GALK1 is a small molecule kinase of the GHMP kinase family, which catalyzes the MgATP-dependent phosphorylation of the C-1 hydroxyl of α-d-galactose to yield Gal-1-P in the Leloir pathway. In classic galactosemia, GALT enzymatic deficiency causes the accumulation of Gal-1-P, the product of the enzyme galactokinase 1 (GALK1; EC 2.7.1.6) upstream of GALT in the Leloir pathway. Inhibition of human GALK1 (hGALK1) to prevent Gal-1-P production therefore could provide a therapeutic benefit for GALT deficiency. Here, we determined crystal structures of hGALK1 bound with reported ATP-competitive inhibitors of the spiro-benzoxazole series, to reveal their binding mode in the active site.

To this end, we co-crystallized hGALK1 with two spiro-benzoxazole inhibitors (T1 and T2), in the presence of galactose, and determined their crystal structures to 2.44 and 2.10 Å resolution, respectively. T1 and T2 share the chemical scaffold of a benzoxazole ring connected to a tetrahydroquinazolinone ring by an amide linker, and both compounds are found to occupy the ATP binding site in a similar manner. The benzoxazole ring, mimicking the adenine moiety of ATP, sits in a hydrophobic pocket forming a π–π stacking interaction with Trp106 and van der Waals interactions with Val129 and Leu145. Importantly, the quinazolinone cyclohexanone and spiro-ring substituents cause displacement of two key side-chains—Arg105 and Arg228—at the entrance of the ATP site. In our costructures, both Arg105 and Arg228 are sequestered away from the ATP phosphate groups, to accommodate the quinazolinone ring of the compounds. For T2 with the larger spiro ring, the carbonyl moiety is close enough to hydrogen bond with the Arg105 guanidino side chain (dotted line). Therefore, these residues are sequestered away from catalysis in the inhibitor-bound complexes. ATP-titration experiments with T2 showed no significant change in Vmaxapp (P = 0.1801) and a significant increase in Kmapp (P < 0.0001), collectively indicating competitive inhibition with ATP by T2, which is supported by fitting in GraphPad Prism and is in agreement with its binding mode in our hGALK1 crystal costructure. We found that hGALK1 co-crystallized with galactose and T2 produced the required quantity (crystals in the hundreds) and diffraction quality (consistently better than 2.5 Å) for the screening campaign. To bias hits toward allosteric binding, we soaked compounds into hGALK1 co-crystals with galactose and T2 occupying the active site.

>HHAALRQPQVAELLAEARRAFREEFGAEPELAVSAPGRVNLIGEHTDYNQGLVLPMALELMTVLVGSPRKDGLVSLLTTSEGADEPQRLQFPLPTAQRSLEPGTPRWANYVKGVIQYYPAAPLPGFSAVVVSSVPLGGGLSSSASLEVATYTFLQQLCPDSGTIAARAQVCQQAEHSFAGMPCGIMDQFISLMGQKGHALLIDCRSLETSLVPLSDPKLAVLITNSNVRHSLASSEYPVRRRQCEEVARALGAASLREVQLEELEAARDLVSKEGFRRARHVVGEIRRTAQAAAALRRGDYRAFGRLMVESHRSLRDDYEVSCPELDQLVEAALAVPGVYGSRMTGGGFGGCTVTLLEASAAPHAMRHIQEHYGGTATFYLSQAADGAKVLCL[2x]DUSP22 is a small phosphatase containing 184 residues, and the sequence contains a catalytic domain as well as an N-terminal myristoylation site. This enzyme is broadly expressed in different tissues and plays important roles in the regulation of signaling pathways, such as inactivating the T cell receptor (TCR) signaling pathway, activating the JNK signaling pathway, and regulating the phosphorylation of focal adhesion kinase (FAK). The phosphatase domain of DUSP22 consists of five twisted β-sheets and six α-helices, and the structural scaffold is similar to that of DUSP3 (VHR), while DUSP22 does not contain an N-terminal α-helix surrounded by the N-loop. In this region, the catalytic activity is facilitated by C88 in the P-loop and D57 in the D-loop, and the hydrogen bonding network is formed by D57 in the D-loop, S93 in the P-loop, and N128 in the N-loop.

Structural alignment among N128A, N128D, and WT_VO4 revealed that N128 participated in forming the conformation of the D-loop. In the N128A structure, one hydrogen bond was formed between the side chain of S93 and the backbone amide of A128. The interaction between D57 and N128 was broken, and no water-mediated hydrogen bonds connected them. The D-loop was shifted away in the N128A mutant, indicating that the hydrogen bond from S93 was not sufficient to stabilize the D-loop. The negative charge from D128 in the N128D mutant induced charge repulsion against D57, which resulted in unclear electron density in the conformation of the D-loop and slightly shifted the N-loop. These results clearly indicated that the N128-D57 interaction anchored the D-loop and stabilized the conformation of the active site. N128A and N128D increased the KM more than 30 times, but the kcat values were different. N128D decreased the kcat by 16 times, while the kcat of N128A only decreased 2.5 times. Disruption of the DPN–triloop interaction by N128A and N128D critically decrease the catalytic efficiency by 100–500 times because it induces conformation changes in the D-loop and perturbs the conformation of the P-loop. N128A does not form a barrier against D57, so D57 can interact with S93 due to D-loop dynamics and catalyze the substrate, while this interaction is not stable and induces a high KM.

> GPMGNGMNKILPGLYIGNFKDARDAEQLSKNKVTHILSVHDSARPMLEGVKYLCIPAADSPSQNLTRHFKESIKFIHECRLRGESCLVHCLAGVSRSVTLVIAYIMTVTDFGWEDALHTVRAGRSCANPAVGFQRQLQEFEKHEVHQYRQWLKEEYG>[4x]HHHHHHAVAKDSTESKSWEPFSLSPIKDPQALHKELCSKNVIPVTSTLEDLLPATQAQHVFIKRGTFHSYNWTIKGRSLNMDRLRETCQSLVDRHSILRTSFVEHEGHPIQLVLANLDVKVREVQCWPGEDPMEVCKALWDG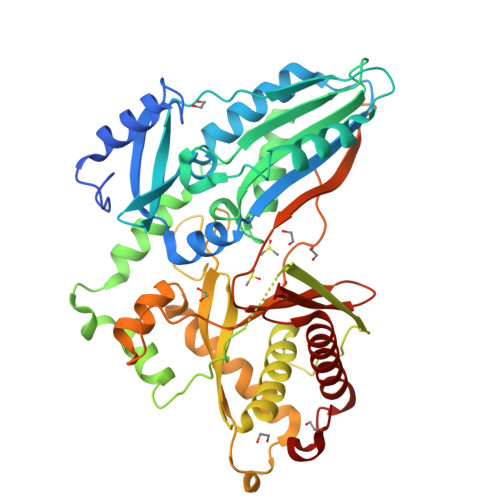KDWPTLNVLGGSLPVRFTLVSCPGNEHVVLTIQISHSQWDGVSIPKLFSDFAAIYNQTPLPPTSDFAHYLYHRVSSAREDVQQDPTFQFWRHYLDGAKMAVPFAPRALTLCAEPAAAAQSGQTLWTFKGIVPPTLPSGITMATLVKAATALFLSYHLGSRDVVFGHTVNGRNLPMDNIESLLGCTLNFVPLRVTFPEDSTDWTVMDLLHHTQTQYTRALSHEHVELRDIFQHSTNWPAETPLSLIVQHQNIDLSFSLPLRGSSLDVQYSKFARFDPLDEVWIFTEPHADRLEVQVCANSRVLGQEQATELANNISAIITKFSTDPTARLLDITF>GSHMEAVQNRIVEAAERVPGVRGVIHLRARYVGQDIWADMIIGVDPENTVEQAHEISEAVQAAVCGKIRRIESLHV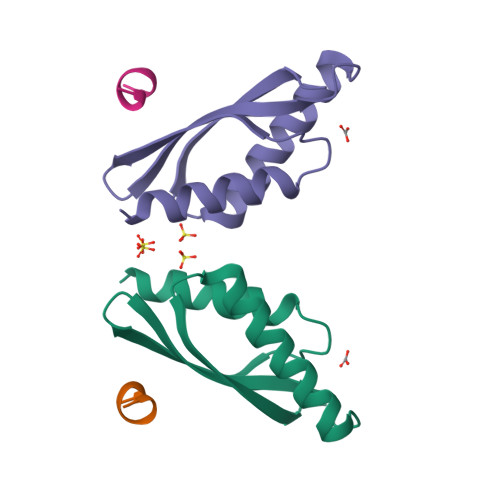SAEAREIGDTTKPSFSDQPLSFDEVMLSKVDN[2x]>[3x]MAANSTRRPIIAFMSDLGTTDDSVAQCKGLMYSICPDVTVVDVCHSMTPWDVEEGARYIVD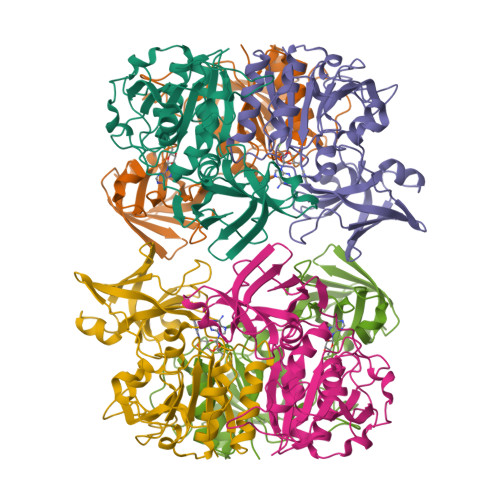LPRFFPEGTVFATTTYPATGTTTRSVAVRIKQAAKGGARGQWAGSGAGFERAEGSYIYIAPNNGLLTTVLEEHGYLEAYEVTSPKVIPEQPEPTFYGREMVAIPSAHLAAGFPLSEVGRPLEDHEIVRFNRPAVEQDGEALVGVVSAIDHPFGNVWTNIHRTDLEKAGIGYGARLRLTLDGVLPFEAPLTPTFADAGEIGNIAIYLNSRGYLSIARNAASLAYPYHLKEGMSARVEAR>[2x]SAIERITKAAHLIDMNDIIREGNPTLRTVAEEVTFPLSDQEIILGEKMMQFLKHSQDPVMAEKMGLRGGV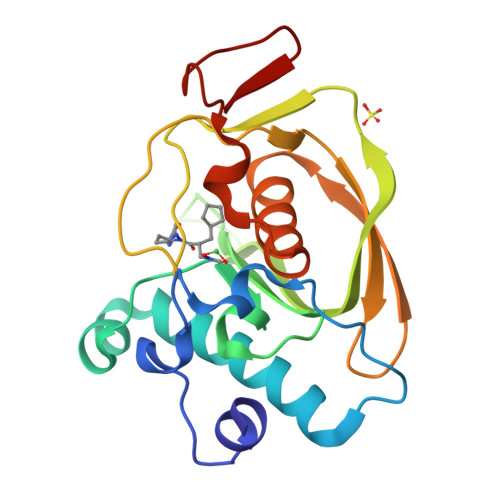GLAAPQLDISKRIIAVLVPNIVEEGETPQEAYDLEAIMYNPKIVSHSVQDAALGEGEGCLSVDRNVPGYVVRHARVTVDYFDKDGEKHRIKLKGYNSIVVQHEIDHINGIMFYDRINEKDPFAVKDGLLILE>NDKLVELSKSDDNWVMPGKNYDSNNFSDLKQINKGNVKQLRPAWTFSTGLLNGHEGAPLVVDGKMYIHTSFPNNTFALGLDDPGTILWQDKPKQNPAARAVACCDLVNRGLAYWPGDGKTPALILKTQLDGNVAALNAETGETVWKVENSDIKVGSTLTIAPYVVKDKVIIGSSGAELGVRGYLTAYDVKTGEQVWRAYATGPDKDLLLASDFNIKNPHYGQKGLGTGTWEGDAWKIGGGTNWGWYAYDPGTNLIYFGTGNPAPWNETMR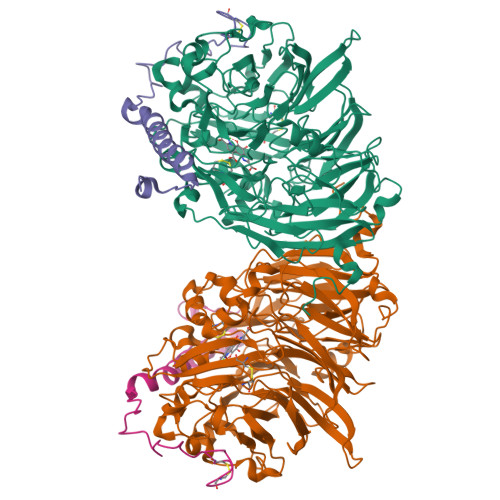PGDNKWTMTIFGRDADTGEAKFGYQKTPHDEWDYAGVNVMMLSEQKDKDGKARKLLTHPDRNGIVYTLDRTDGALVSANKLDDTVNVFKSVDLKTGQPVRDPEYGTRMDHLAKDICPSAMGYHNQGHDSYDPKRELFFMGINHICMDWEPFMLPYRAGQFFVGATLNMYPGPKGDRQNYEGLGQIKAYNAITGDYKWEKMERFAVWGGTMATAGDLVFYGTLDGYLKARDSDTGDLLWKFKIPSGAIGYPMTYTHKGTQYVAIYYGVGGWPGVGLVFDLADPTAGLGAVGAFKKLANYTQMGGGVVVFSLDGKGPYDDPNVGEWKSAAK[2x];>[2x]YDGTKCKAAGNCWEPKPGFPEKIAGSKYDPKHDPKELNKQADSIKQMEERNKKRVENFKKTGKFEYDVAKISAN> MAPTPKYTFTERAAAGNLSDAEILNSNNPTGSELPDESDVVVGGAGIHGLIYALHASKYKPNNLKISVIEKNTRPGYKIGESTLPIFYTWCKLHGISAAYLLRLFGLKDGLCFYFLDRENQGQYTDFCSVGAPGLVLASLQIERPMSELLFTILAQRNGVNVYHGREVDFKSTVVQGGGQGNKIAVSRGKYDSTPKTIDSALFVDATGRFRQFCSKKAPRHRFDGWNCNAFWGYFTAPKDESKIPFDLYEGDHTNHLCFPEGWVWVIRLPSWEGSPIANLMDMVTYILECADAGVPGDELPSSEELARMFGLKFQWVTSIGFAVRNDVKYPEDLSAYGTREAEQKFNYFVQKYELLQQFMSNFELIENLYGPGTTWFIRKTLAYQSPVVSGPG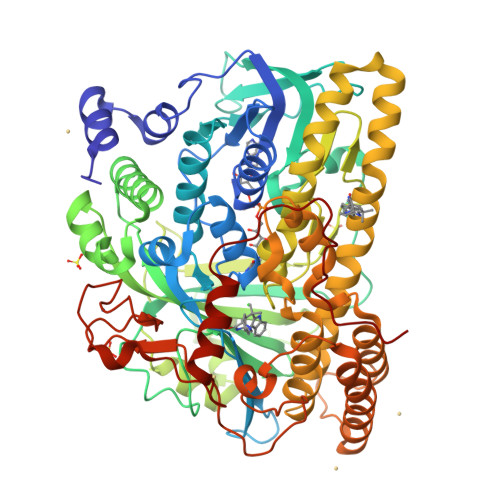WLAIGDACGFTNPLYSPGINVGMSTSTWAAQLSHPIVEIGKSAPADAAESSIRKLLVPYDDYCKSLVPALEQMNRFNYVCYRDTRLGPQVACLWQFFAGIERYLSDVNIETFAHYAIKWVWGAMVPEYQQVAQKCIEHIETVPLDERLPDAMVDELLAFSNRIKSAAVAADDFSLRWDAILRSFDRSLNFVEGKTSRDIYTRQCSGCGAWLQLRPDWKKCHSCGLLGTEPQTAVTFDPPLTAEEEALLYAAWNTAPKYDPSKELKLPTPTRPAA>[4x]EDPPACGSIVPRREWRALA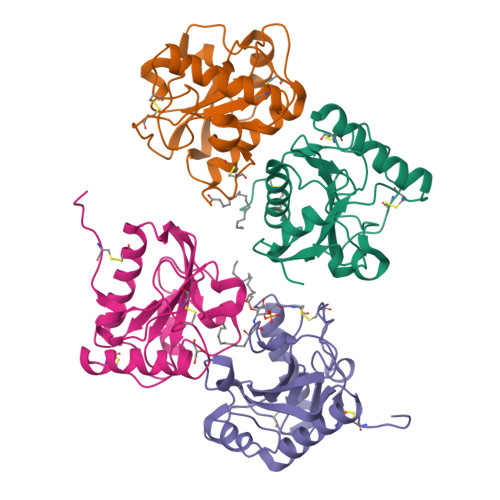SECRERLTRPVRYVVVSHTAGSHCDTPASCAQQAQNVQSYHVRNLGWCDVGYNFLIGEDGLVYEGRGWNIKGAHAGPTWNPISIGISFMGNYMNRVPPPRALRAAQNLLACGVALGALRSNYEVKGHRDVQPTLSPGDRLYEIIQTWSHYRA Herein we have characterized the structural, biophysical, and biochemical properties of the first enzyme (d-lactate dehydrogenase [d-LDH]; TP0037) predicted in this pathway. Binding and enzymatic studies showed that recombinant TP0037 consumed d-lactate and NAD+ to produce pyruvate and NADH. The crystal structure of TP0037 revealed a fold similar to that of other d-acid dehydrogenases; residues in the cofactor-binding and active sites were homologous to those of other known d-LDHs. The crystal structure and solution biophysical experiments revealed the protein’s propensity to dimerize, akin to other d-LDHs.

The protein yielded crystals that diffracted well, and molecular-replacement phasing followed by standard refinement approaches resulted in a model for the protein at a resolution at 1.38 Å. The difference electron-density maps associated with this structure were carefully scrutinized for evidence of any bound substrates or cofactors, but the only convincing densities were assigned to solutes in the crystallization medium (ethylene glycol and chloride ion). We hence considered the structure to be the unliganded or an “apo” form of the protein. The TP0037 crystal structure featured two domains with a cleft between them. The smaller domain which, by convention, we termed the “C” domain (“C” being an abbreviation for “catalytic”), comprised a central β-sheet flanked by α-helices. The second, larger domain, termed the NB domain (NB for “nucleotide-binding”) because of its role in binding the nucleotide-based cofactor NAD+ (or NADH), harbored a centrally located seven-strand parallel β-sheet. The interface between the monomers was formed almost entirely by the respective NB domains such that the two C domains were found on opposite ends of the dimer. The NB domain protuberances noted above figured prominently in the intermolecular contacts, reaching across the dimeric interface and interacting with each other. E264, H296, and R235 were the structural homologs of these amino acids in TP0037, and they adopted similar relative positions in the putative active site of the treponemal protein. Hence, the structure of TP0037 revealed that parts of the interdomain cleft closely resembled both the cofactor-binding site and the active site of a known d-lactate dehydrogenase (LbD-LDH).

>[2x]GAMGSMRCVVFNLREEEAPYVEKWKQSHPGVVVDTYEEPLTAKNKELLKGYEGLVVMQFLAMEDEVYDYMGACKLKVLSTRTAGFDMYNATLLKKHGIRLTNVPSYSPNAIGEYALAAALQLTRHAREIETFVRKRDFRWQKPILSKELRCSRVGILGTGRIGQAAARLFKGVGAQVVGFDPYPNDAAKEWLTYVSMDELLSTSDVISLHMPATKDSHHLINAKTIAQMKDGVYLVNTARGAVIDSQALLDSLDKGKIAGAALDAYEFEGPYIPKDNGNNPITDTVYARLVAHERIIYTPHIAFYTETAIENMVFNSLDACTTVLRGEPCAAEIKL2'-deoxy-5-{(1E)-5-[(10-hydroxydecanoyl)amino]pent-1-en-1-yl}uridine 5'-(tetrahydrogen triphosphate) | C24 H42 N3 O16 P3 | 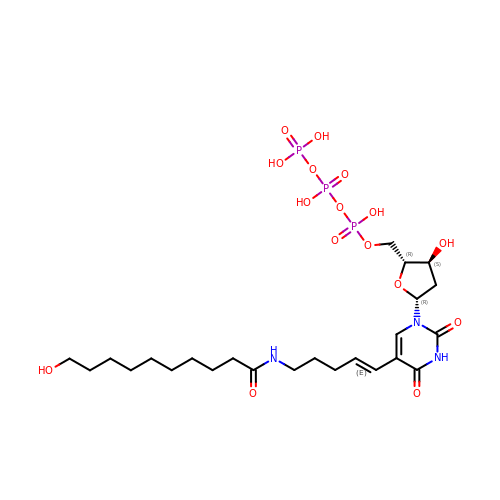YHNZXWUFXLSXJT-GJAYGDSISA-N> STCDDEPIHIPGAIQPHGLLLALAADMTIVAGSDNLPELTGLAIGALIGRSAADVFDSETHNRLTIALAEPGAAVGAPITVGFTMRKDAGFIGSWHRHDQLIFLELEPPQRDVAEPQAFFRHTNSAIRRLQAAETLESACAAAAQEVRKITGFDRVMIYRFASDFSGEVIAEDRCAEVESKLGQHYPASDIPAQAR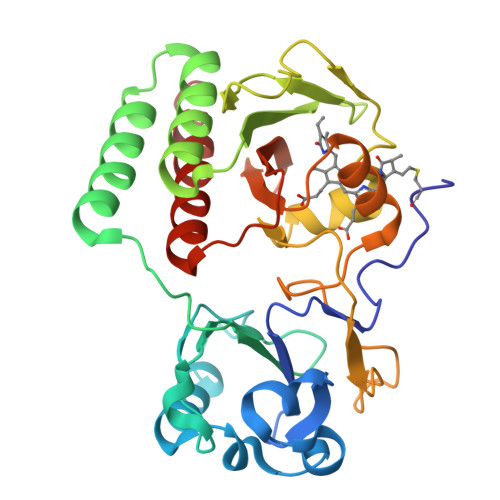RLYTINPVRIIPDINYRPVPVTPDLNPVTGRPIDLSFAILRSVSPVHLEFMRNIGMHGTMSISILRGERLWGLIVCHHRTPYYVDLDGRQACELVAQVLARAIGVMEE> MKKYTCTVCGYIYNPEDGDPDNGVNPGTDFKDIP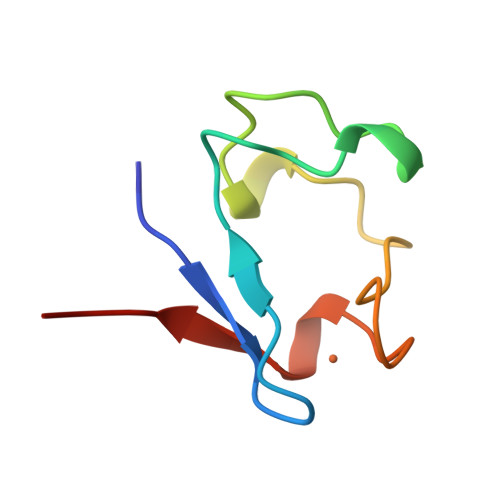DDWVCPLCAVGKDQFEEVEE> MAPLQPGDSFPANVVFSYIPPTGSLDLTVCGRPIEYNASEALAKGTSVLVAV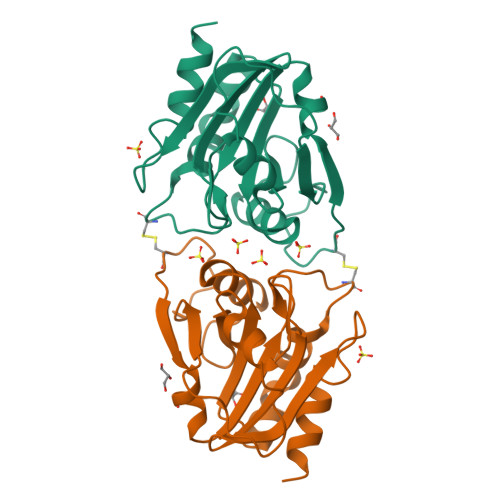PGAFTPTCQEKHVTGFIAKLDQLRQAGVDRVLFIASNDAFVMSAWGKANGIKDESILFLSDSDTAFSSSIGWANAGRTGRYAIVVKDGKVVYAAVDTVRGSTEKSGVDAVLTVLGNQGKL> GSHGGIEGVKGAASGVVGELARARLALDERGQKLSDLEERTAA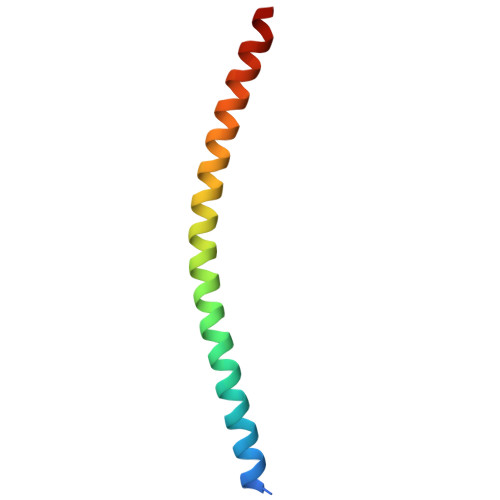MMSSADSFSKHAHEMMLKYK>[4x]MKILVIEDDALLLQGLILAMQSEGYVCDGVSTAHEAALSLASNHYSLIVLDLGLPDEDGLHFLSRMRREKMTQPVLILTARDTLEDRISGLDTGADDYLVKPFALEELNARIRALLRRHNN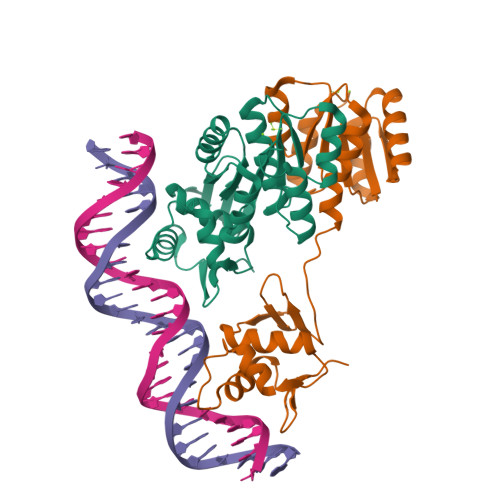QGDNEISVGNLRLNVTRRLVWLGETALDLTPKEYALLSRLMMKAGSPVHREILYNDIYSGDNEPATNTLEVHIHNLREKIGKSRIRTVRGFGYMLANNDDTEHLEHHHHHH>MNHKVHHHHHHLQENLYFQGMGAEPQQLHVVFFPIMAHGHMIPTLDIARLFAARNVRATIITTPLNAHTFTKAIEMGKKNGSPTIHLELFKFPAQDVGLPEGCENLEQALGSSLIEKFFKGVGLLREQLEAYLEKTRPNCLVADMFFPWATDSAAKFNIPRLVFHGTSFFSLCALEVVRLYEPHKNVSSDEELFSLPLFPHDIKMMRLQLPEDVWKHEKAEGKTRLKLIKESELKSYGVIVNSFYELEPNYAEFFRKELGRRAWNIGPVSLCNRSTEDKAQRGKQTSIDEHECLKWLNSKKKNSVIYICFGSTAHQIAPQLYEIAMALEASGQEFIWVVRNNNNNDDDDDDSWLPRGFEQRVEGKGLIIRGWAPQVLILEHEAIGAFVTHCGWNSTLEGITAGVPMVTWPIFAEQFYNEKLVNQILKIGVPVGANKWSRETSIEDVIKKDAIEKALREIMVGDEAEERRSRAKKLKEMAWKAVEEGGSSYSDL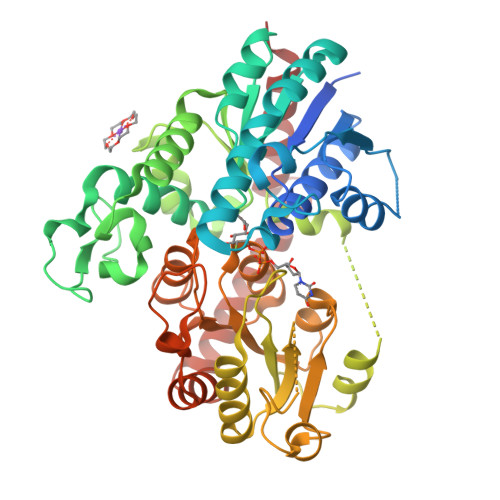SALIEELRGYHA[2x]>[2x]MASGSASSAQTPGLMSWLPPSNQLSPEARSVLDRMDAAKAPEFNGDLVRQRAFYQQFNDDRLVEMRRVFRTRERHETLNAVHVQVVEPADGVSARNRDRVLINVHGGAFMWGAGSGALVEAIPIAATMGVSVVTVDYRLAPENRYPAASEDVTAVYRALLERYPAANIGIFGCSAGGVITAQAVTWIRREG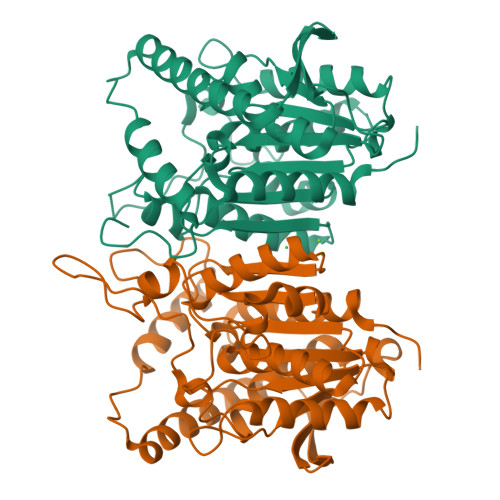LPRPGAIGTLCGTGAPYSGDSPYLAGVVPVGPGVKAPPLPGLLPTAYMEGVGADDARAYPLTSDAETVFMPPTLLLAGGRDFAVSALSLAHRRLARAGVDSELHLFDGLPHAFFVWPDMPESLEAYALIAGFFDSRLGLTPSSSIPTPRSPSHHHHHH> GPMARTFILWLHGLGDSGPANEPIQTQFKSSELSNASWLFPSAPFNPVTCNNGAVMRSWFDVPELPFKVGSPIDESSVLEAVKNVHAIIDQEIAEGTNPENVFICGLSQGGALTLASVLLYPKTLGGGAVLSGWVP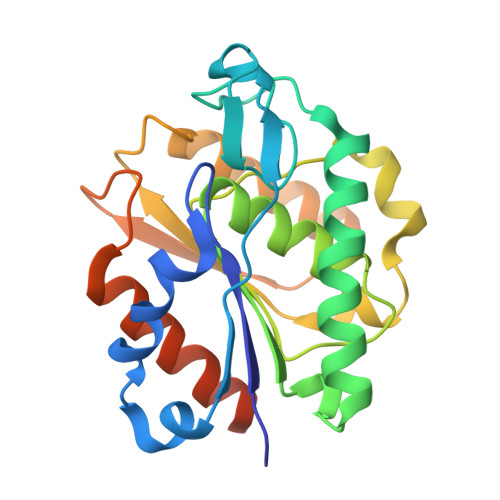FTSSIISQFPEEAKKTPILWSHGTDDRMVLFEAGQAALPFLKEAGVTCEFKAYPGLGHSISNKELKYIESWIKRRLKGSSSTCLQLNCLKEMFH>[3x]SQQFNVAIFGATGAVGETMLEVLQEREFPVDELFLLASERSEGKTYRFNGKTVRVQNVEEFDWSQVHIALFSAGGELSAKWAPIAAEAGVVVIDNTSHFRYDYDIPLVVPEVNPEAIAEFRNRNIIANPNCSTIQMLVALKPIYDAVGIERINVTTYQSVSGAGKAGI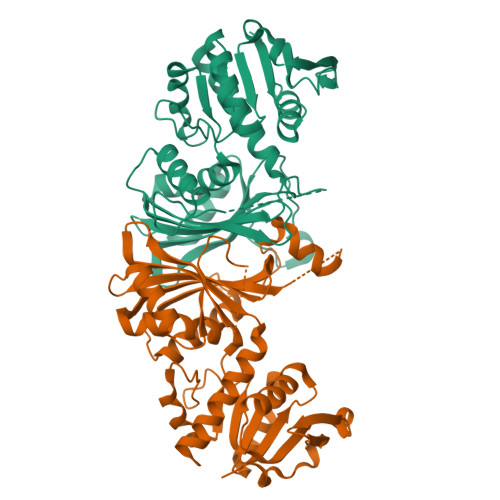DELAGQTAKLLNGYPAETNTFSQQIAFNCIPQIDQFMDNGYTKEEMKMVWETQKIFNDPSIMVNPTCVRVPVFYGHAEAVHVETRAPIDAEQVMDMLEQTDGIELFRGADFPTQVRDAGGKDHVLVGRVRNDISHHSGINLWVVADNVRKGAATNAVQIAELLVRDYF> MASMTGGQQMGRDEAGITGTWYNQLGSTFIVTAGADGALTGTYESAAGKAESRYVLTGRYDSAPATDGSGTALGWTVAWKNNYRNAHSATTWSGQYVGGAEARINTQWLLTSGQTEA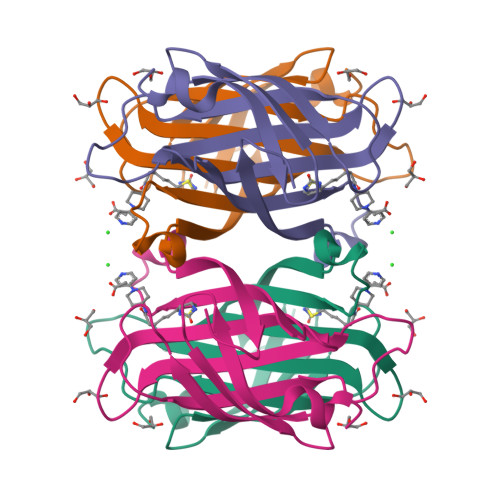NGWRSTLVGHDTFTKVKPSAASIDAAKKAGVNNGNPLDAVQQ> GDPKEEEEEEEELVDPLTTVREQCEQLEKCVKARERLELCDERVSS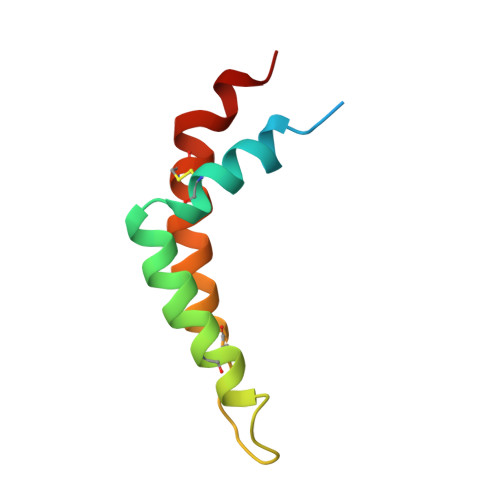RSQTEEDCTEELFDFLHARDHCVAHKLFNSLK Template-independent terminal ribonucleotide transferases (TENTs) catalyze the addition of nucleotide monophosphates to the 3′-end of RNA molecules regulating their fate. TENTs include poly(U) polymerases (PUPs) with a subgroup of 3′ CUCU-tagging enzymes, such as CutA in Aspergillus nidulans. CutA preferentially incorporates cytosines, processively polymerizes only adenosines and does not incorporate or extend guanosines. Here, we report structures of the catalytic core of T. terrestris CutA (TtCutA) in the apo form and its complexes with a non-hydrolyzable CTP analog and A3 RNA.

The other crystal was CutA in complex with an A3 RNA oligonucleotide, which was obtained by soaking crystals of apo protein crystals with RNA. This structure was solved to 1.9 Å resolution and refined to an Rfree of 21.3%. In the CutA–A3 complex structure, the 3′-terminal nucleotide of the RNA occupies the position of the incoming nucleotide. Therefore, it represents a product complex that forms after incorporation of the nucleotide but before translocation of the RNA to allow binding of the next incoming nucleotide. In this structure, a single Mg2+ ion is observed that is located closer to the position of the divalent metal ion A from the canonical fully formed polymerase active site. This metal ion interacts with Asp341 and the phosphate group between the last and penultimate nucleotide of the RNA. The 2′-OH group of nt −1 forms a hydrogen bond with Asp341, which also participates in coordination of the catalytic metal ion at the active site. The base edge (imine nitrogen N1) is hydrogen-bonded with a side chain of Asn397. The exposed 5′-side surface of the base forms van der Waals interactions with the side chain of Val377. The third nucleotide of the RNA in the CutA-A3 complex (nt −2) is located in a narrow cleft between the finger and palm subdomains.

>[4x]ETAIPFSRRRMPYSLGTDKLEKVDPDKIKSKLSEDVERKLETDMRELYDRLLPTEAIEVNRRELVSKLERLFNTEWPGHDIRVHLFGSSGNLLCSDDSDVDICITTPWRELESVCMIAELLDRHGMEKVVCVSSAKVPIVKIWDPELKLACDMNVNNTLALENTRMVRTYVSIDDRVRPLAMIIKYWTRRRVVNDAAFGGTLSSYTWICMIIAFLQLRDPPVLPALHQQHDLKLVKQDGALSDFADDIPKLRGFGAKNKDSLAVLLFQFFRFYAHEFDYDKYTLSIRMGTLLTKAEKNWQYLVNNALCVEEPFNDGRNLGNTADETSFRGLHMELRRAFDLIAEGKLEECCEQYVFPKEEERV~{N}-[4-[2,4-bis(fluoranyl)phenoxy]-3-[2-(1~{H}-imidazol-5-yl)-5-methyl-4-oxidanylidene-furo[3,2-c]pyridin-7-yl]phenyl]ethanesulfonamide 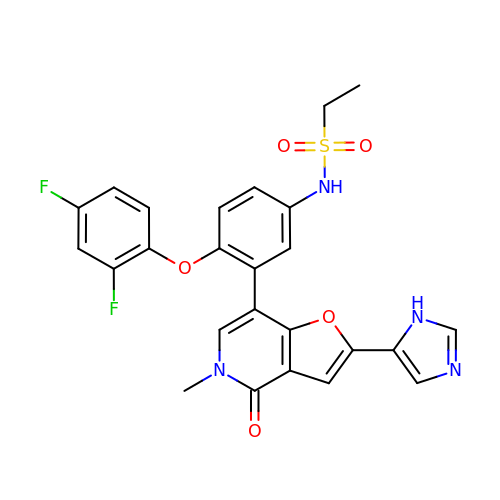| C25 H20 F2 N4 O5 S | BWALAYQEQUFOGH-UHFFFAOYSA-N> MRVKHYIQREFNYSVSSQDLLDIATRIAISAIKPKPKSNKPEPYVDSSTINSLLSFLQSRRNVNELLLYIMRQAGRDEIDEETGKL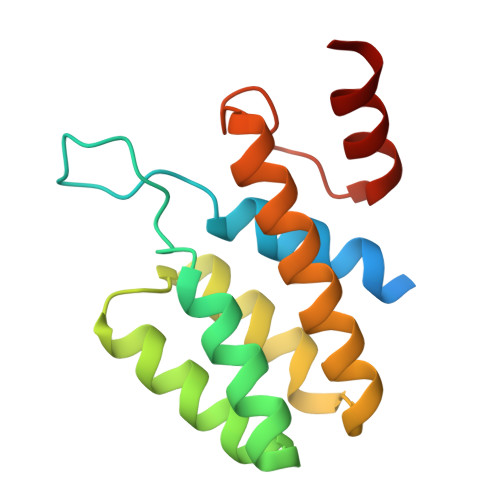LLASLKDRELKDAVNLLGYVKWVYDTLTGLKVNYNNVKGVKTFKELVNILSKV The SARS-CoV-2 N protein binds to viral genomic RNA and oligomerizes around it to form a closed capsule that both protects the genome from antiviral responses and directs its packaging into new virions. Beyond its role in nucleocapsid assembly and packaging, the N protein is also important during viral RNA synthesis, where it binds double-stranded RNA during viral genome replication and participates in the discontinuous transcription process necessary to generate subgenomic mRNAs. The protein is comprised of five domains. There are two stable, proteolysis-resistant domains, the N-terminal RNA binding domain (N-RBD), which binds to virus genomic RNA, and the dimerization domain (N-DD), which facilitates protein oligomerization and has some nonspecific RNA binding activity.

We determined the first publicly available structure of SARS-CoV-2 N-DD (residues 247 to 364), which was released on 22 April 2020 to the Protein Data Bank with accession no. The crystal belonged to the P212121 space group (cell parameters, a = 43.61, b = 122.32, c = 130.63) and was refined to 2.05 Å resolution. The asymmetric unit consisted of six polypeptide chains, which formed three homodimers. Each protomer contained 108 residues (257 to 364) that formed 5 α helices, α1 (269 to 275), α2 (288 to 295), α3 (301 to 306), α4 (310 to 318), and α5 (345 to 357); 3 η helices, η1 (258 to 262), η2 (296 to 298), and η3 (358 to 363); and 2 β-strands, β1 (319 to 325) and β2 (328 to 338), all of which were connected by five loops. The SARS-CoV-2 N-DD homodimer resembles a rectangular prism with a buried surface area of ~5,274 Å2. One large interface is formed by a four-stranded, antiparallel β-sheet, comprised of the paired protomer β-hairpins (β1-β2–β′1-β′2) (best depicted between chains A and B). A second large interface is formed by interlocked helices and loops (α4-η′1) (best depicted between chains C and D). The structure has nine chloride ions bound, which were positioned on the positively charged helical face of each dimer. The overall topology observed in our structure was essentially identical to the 13 subsequently deposited structures of the SARS-CoV-2 N-DD. In the N-DD, the immunogenic peptides mapped to regions that projected away from the dimer interface and thus are exposed even in the dimerized form.

>[6x]SNATKKSAAEASKKPRQKRTATKAYNVTQAFGRRGPEQTQGNFGDQELIRQGTDYKHWPQIAQFAPSASAFFGMSRIGMEVTPSGTWLTYTGAIKLDDKDPNFKDQVILLNKHIDAYKTFP N-(4-methyl-1,3-thiazol-2-yl)oxane-4-carboxamide 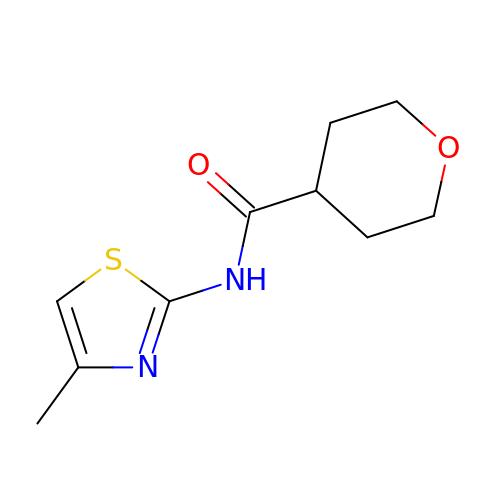| C10 H14 N2 O2 S | QIRPROGVHFZLPG-UHFFFAOYSA-N>INQVRPKLPLLKILHAAGAQGEMFTVKEVMHYLGQYIMVKQLYDAAAQHMVYCGGDLLGELLGRQSF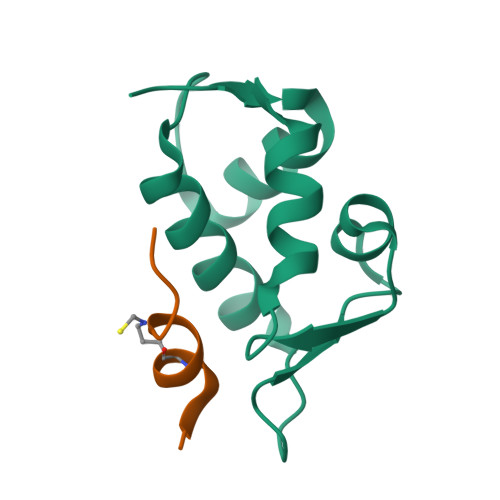SVKDPSPLYDMLRKNLVT[8x];>XTSFKEYWCLLSPX[8x]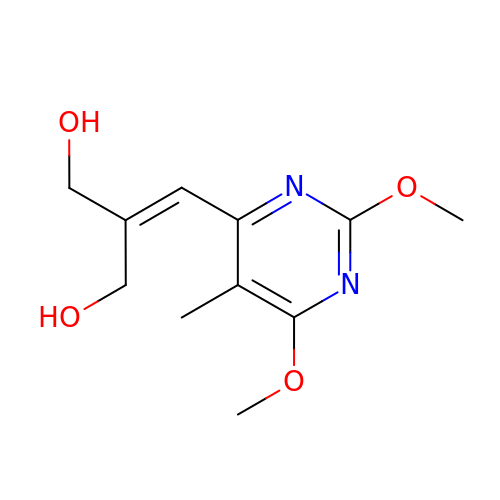2-[(2,6-dimethoxy-5-methylpyrimidin-4-yl)methylidene]propane-1,3-diol | C11 H16 N2 O4 | YLFWDZOXQQHLDL-UHFFFAOYSA-N>MKGYGEMAKNNPTRITAEPGKQEIIITREFDAPRELVFKAFTDPDLYTQWIGPRGFTTALKIFEPKNGGSWQYIQKDPEGNEYAFHGVNHDVTEPERIISTFEFEGLPEKGHVILDTARFEALPGDRTKLTSHSVFQTIEDRDGMLQSGMEEGINDSYERLDELLEKMKKLEHHHHHH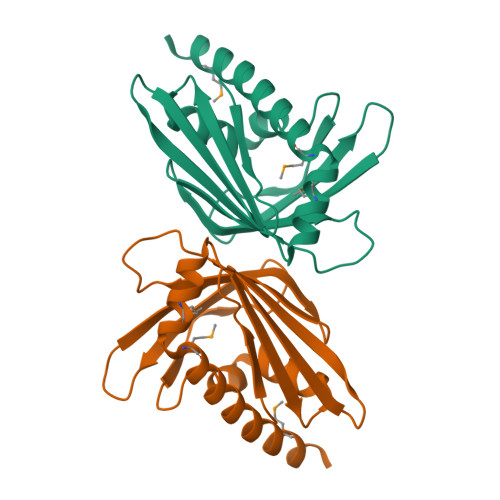[3x]> MALLGTILLPLLGFALLGLFGKRMREPLPGVLASGLVLASFLLGAGLLLSGGARFQAEWLPGIPFSLLLDNLSGFMLLIVTGVGFLIHVYAIGYMGGDPGYSRFFAYFNLFIAMMLTLVLADSYPVMFIGWEGVGLASFLLIGFWYKNPQYADSARKAFIVNRIGDLGFMLGMAILWALYGTLSISELKEAMEGPLKNPDLLALAGLLLFLGAVGKSAQIPLMVWLPDAMAGPTPVSALIHAATMVTAGVYLIARSSFLYSVLPDVSYAIAVVGLLTAAYGALSAFGQTDIKKIVAYSTISQLGYMFLAAGVGAYWVALFHVFTHAFF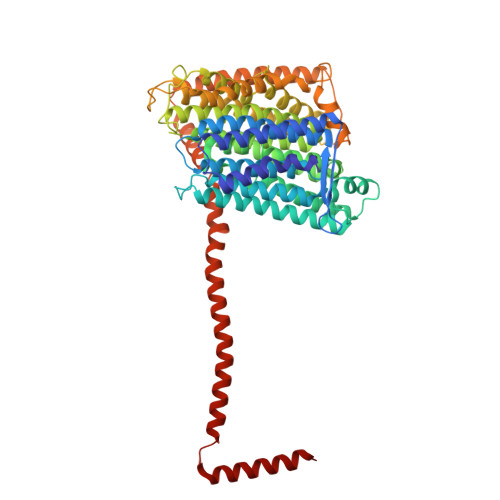KALLFLASGSVIHALGGEQDVRKMGGLWKHLPQTRWHALIGALALGGLPLLSGFWSKDAILAATLTYPFGGVGFYVGALLVAVLTAMYAMRWFVLVFLGEERGHHHPHEAPPVMLWPNHLLALGSVLAGYLALPHPLPNVLEPFLKPALAEVEAHHLSLGAEWGLIALSAAVALLGLWAGFVFFQRKVFPAWYLAFEAASREAFYVDRAYNALIVNPLKALAEALFYGDRGLLSGYFGLGGAARSLGQGLARLQTGYLRVYALLFVLGALLLLGVMRW> DDPPATVYRYDSRPPEDVFQNGFTAWG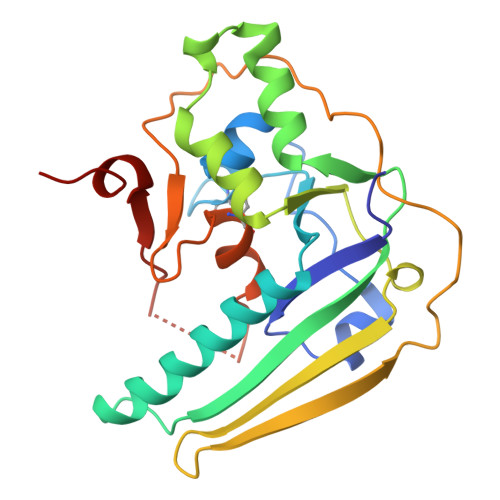NNDNVLEHLTGRSCQVGSSNSAFVSTSSSRRYTEVYLEHRMQEAVEAERAGRGTGHFIGYIYEVRADNNFYGAASSYFEYVDTYGDNAGRILAGALATYQSEYLAHRRIPPENIRRVTRVYHNGITGETTTTEYSNARYVSQQTRANPNPYTSRRSVASIVGTLVRMAPVVGACMARQAESSEAMAAWSERAGEAMVLVYYESIAYSF5-[(3~{R},5~{S})-3-azanyl-5-(trifluoromethyl)piperidin-1-yl]quinoline-8-carbonitrile | C16 H15 F3 N4 | 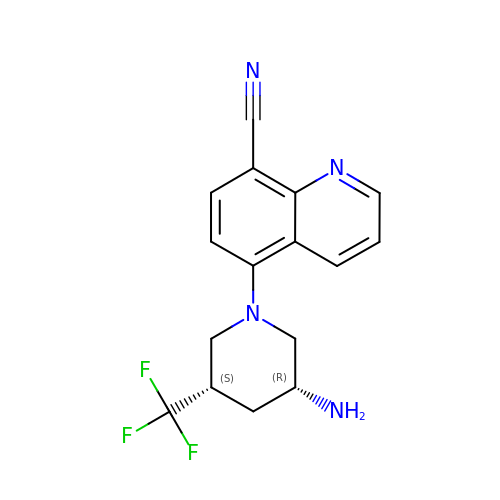BJXYHBKEQFQVES-NWDGAFQWSA-N> SNAMTNRYTTLFA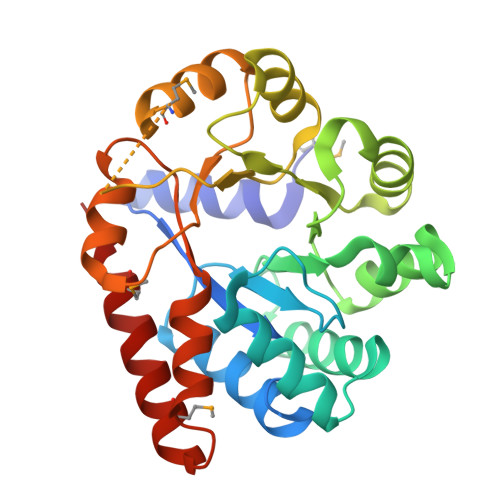NLEKRNEGAFIPFVTIGDPNKALSFEIIDTLVSSGADALELGIPFSDPLADGPTIQEANIRALESGITPKDCFDILTKIRAKYPHIPIGLLLYANLVYANGIENFYQKCLDAGVDSILIADVPAHESKEFRDIAKKVGIAQIFIAPPDASESTLKQISELGSGYTYLLSRVGVTGTETAANMPVEDVLTKLREYNAPKPVLGFGISKPEQVQQAIKAGAAGAISGSATVKIIQNNISNKQKMLNELTYFVKEMKAATLN> GSLVDDKVLVSELIGVDPNPFTQRIMIDKGENDGVFVGQPVLDASGLMGQVVEVMPYTARVLLLTDTTHSIPVQVNRNGLRAIAVGTGNPERLELRYVADTADIKEGDLLVSSGLGQRFPAGYPVATVKEV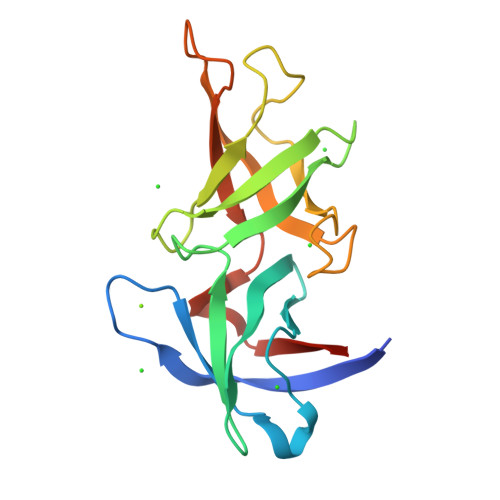IHDSGQPFAVVRAVPTAKMNRSRYVLLVFSDSR>[2x]EPAFNYAEALQKSMFFYEAQRSGKLPENNRVSWRGDSGLNDGADVGLDLTGGWYDAGDHVKFGFPMAFTATMLAWGAIESPEGYIRSGQMPYLKDNLRWVNDYFIKAHPSPNVLYVQVGDGDADHKWWGPAEVMPMERPSFKVDPSC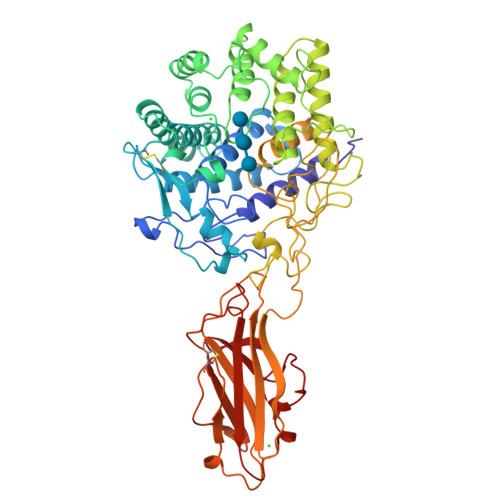PGSDVAAETAAAMAASSIVFADDDPAYAATLVQHAKQLYTFADTYRGVYSDCVPAGAFYNSWSGYQDELVWGAYWLYKATGDDSYLAKAEYEYDFLSTEQQTDLRSYRWTIAWDDKSYGTYVLLAKETGKQKYIDDANRWLDYWTVGVNGQRVPYSPGGMAVLDTWGALRYAANTAFVALVYAKVIDDPVRKQRYHDFAVRQINYALGDNPRNSSYVVGFGNNPPRNPHHRTAHGSWTDSIASPAENRHVLYGALVGGPGSPNDAYTDDRQDYVANEVATDYNAGFSSALAMLVEEYGGTPLADFPPTEEPDGPEIFVEAQINTPGTTFTEIKAMIRNQSGWPARMLDKGTFRYWFTLDEGVDPADITVSSAYNQCATPEDVHHVSGDLYYVEIDCTGEKIFPGGQSEHRREVQFRIAGGPGWDPSNDWSFQGIGNELAPAPYIVLYDDGVPVWGTAP>[4x]MTTRTTDNPWLDARVLNMAHAGGENEAPANTLYAFKRAVKLGANMLELDVQSTKDDQLVVIHNATVDQTTDGTGKVRDLTFEQVHELDAAYNFIPGRHAVPGEPPESYPLRGVRTGEKKPPPGYQPSDFAIPKLADVLEAFPRTPINIEIKGTSDADIPSFLHNAKLLARLLKKTGRTDFIVTSLNDLAVAKFHL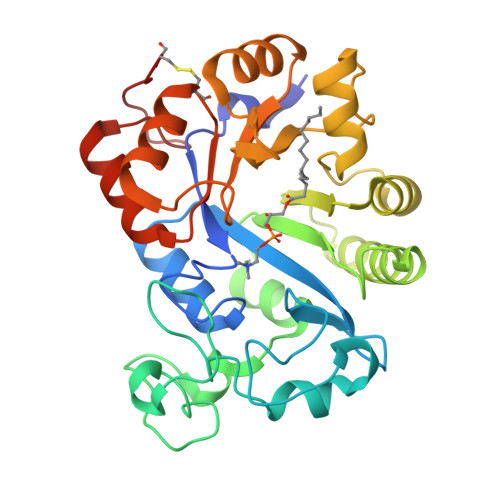LAPDIPIAPGMAGLAAYFLLGVKPMHGTVALQIPVRYQGLEIATPEFIRRAHADGYAVHVWFSGTAPDDEATYNRIIDSCADGLMPAYPALLERILDERGIERPGRPGVDPCGHHHHHH> NVVTDEPKTDKDVKKLGQDDAGYTIGEEFKWFLKSTIPANLGDYEKFEITDKFADGLTYKSVGKIKIGSKTLNRDEHYTIDEPTVDNQNTLKITFKPEKFKEIAELLKGMTLVKNQDALDKATANTDDAAFLEIPVASTINEKAVLGKAIENTFE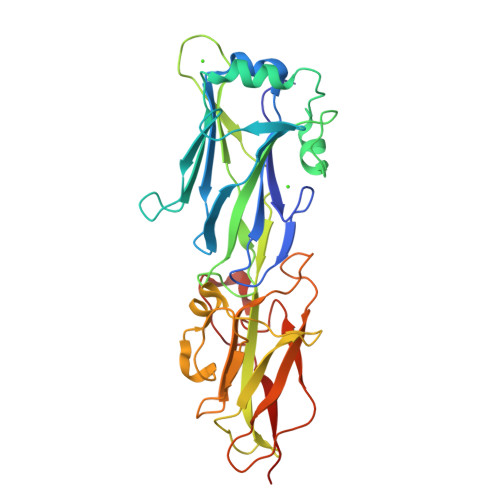LQYDHTPDKADNPKPSNPPRKPEVHTGGKRFVKKDSTETQTLGGAEFDLLASDGTAVKWTDALIKANTNKNYIAGEAVTGQPIKLKSHTDGTFEIKGLAYAVDANAEGTAVTYKLKETKAPEGYVIPDKEIEFTVSQTSYNTKPTDITVDSADATPDTIKNNKR> MAFQILLNLVIAVIWVNFQNSYTAVDFLIGYVVGIFILFVLRRFLRFDFYMRRVWAIIKLIVLFFKELILANIDVIKIV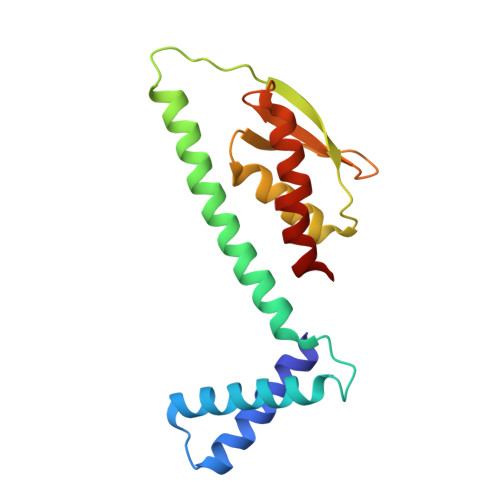LSPKMNIQPGIVAVPTKLKTDWELSLLASLISLTPGTLSMDFSDDNKYIYIHAIDVPNKEKMIRDIHDTFERAILEVTN> MLLEEVCVGDRLSGAAARGDVQEVRRLLHRELVHPDALNRFGKTALQVMMFGSPAVALELLKQGASPNVQDASGTSPVHDAARTGFLDTLKVLVEHGADVNALDSTGSLPIHLAIREGHSSVVSFLAPESDLHHRDASGLTPLELARQRGAQNLMDILQGHMM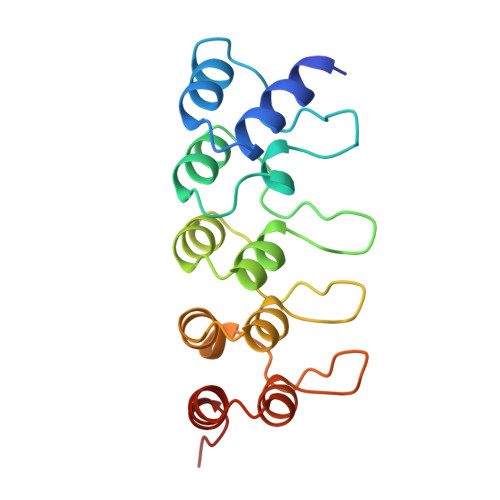IPM>MAIILPDLPYAYDALEPYIDAETMTLHHDKHHATYVANANAALEKHPEIGEDLEALLADVEKIPADIRQALINNGGGHLNHALFWELLSPEKQEPTAEVAAAINEAFGSFEAFQEVFTTSATTRFGSGWAWLVVNAEGKLEVVSTPNQDTPISDGKKPILALDVWEHAYYLKY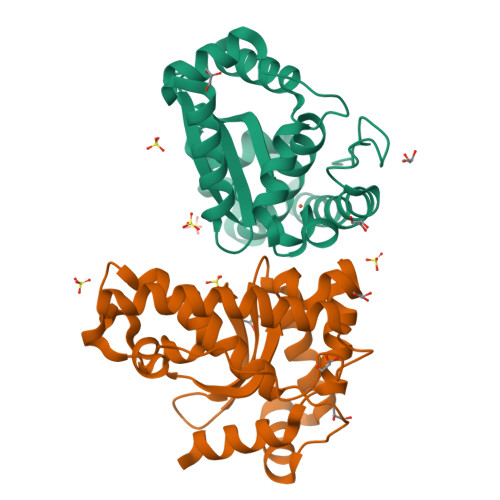RNVRPNYIKAFFEIINWNKVAELYAEALEHHHHHH[2x]>DEPGVATGNGQPVTGNWLAGASQGDGVPIPSQIADQLRGKEFKSWRDFREQFWMAVSKDPSALENLSPSNRYFVSQGLAPYAVPEEHLGSKEKFEIHHVVPLESG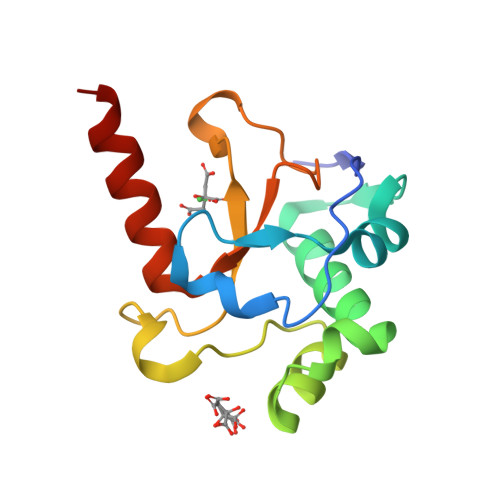GALYNIDNLVIVTPKRHSEIHKELKLKRKEK[2x]>[8x]MLKGFLSTMSPAVRRNKISLIGAGNIGGVMAYLAQLKELGDVVLFDIAPKLGEAKALDIMHANAIYDTAHKAIGTANYEDIADSDVCIITAGLAKLPNKKDEEWSRDDLVAPNSKIMFTIGDNIKKYAPNAFVICITNPLDVMVKMLLKATGFPKNKVVGMGG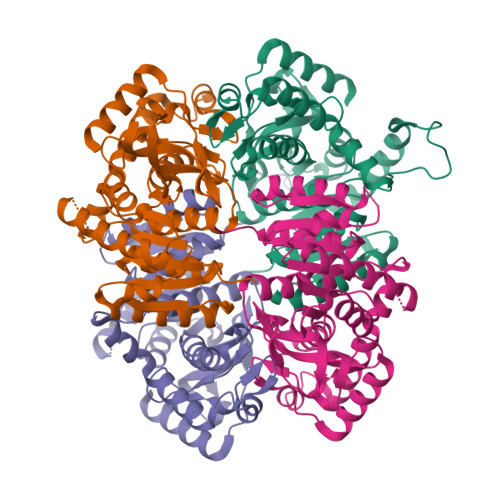LLDSSRMCHYIADKLNVNPRYVHGSCIGGHGDSMIPLVNHVTVNGIPIQLFVERGDITQAELDKIAQRTIGSGMELVQLYGNGSAYFAPATAAIEMASAYLNDKKSVIVCSCYLEGEYGHSDVYLGTPAIIGANGIEKIITLKLSSEEQAKLDASVKEIMRLEALAG> ADPCDLPQTHSLGSRRTLMLLAQMRRISLFSCLKDRHDFGF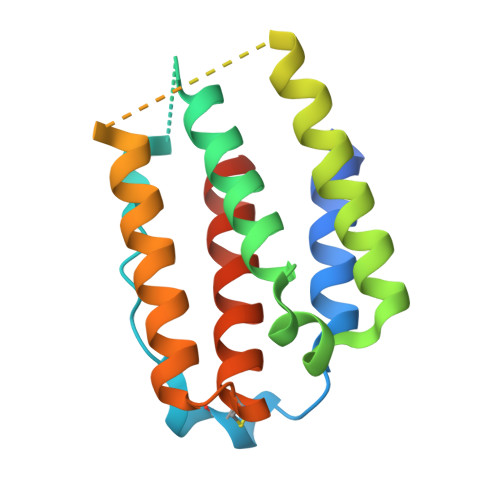PQEEFGNQFQKAETIPVLAAMIAQIFNLFSTKDSSAAWDETLLDKFYTELYQQLNDLEACVIQGVGVTETPLMKEDSILAVRKYFQRITLYLKEKKYSPCAWEVVRAEIMRSFSLSTNLQESLRSKE> MKSKFKLTTAAAMLGLMVLAGGAQAQDKPREVLTGGHSVSAPQENRIYVMDSVFMHLTESRVHVYDYTNGKFLGMVPTAFNGHVQVSNDGKKIYTMTTYHERITRGKRSDVVEVWDADKLTFEKEISLPPKRVQGLNYDGLFRQTTDGKFIVLQNASPATSIGIVDVAKGDYVEDVTAAAGCWSVIPQPNRPRSFMTICGDGGLLTINLGEDGKVASQSRSKQMFSVKDDPIFIAPALDKDKAHFVSYYGNVYSADFSGDEVKVDGPWSLLNDEDKAKNWVPG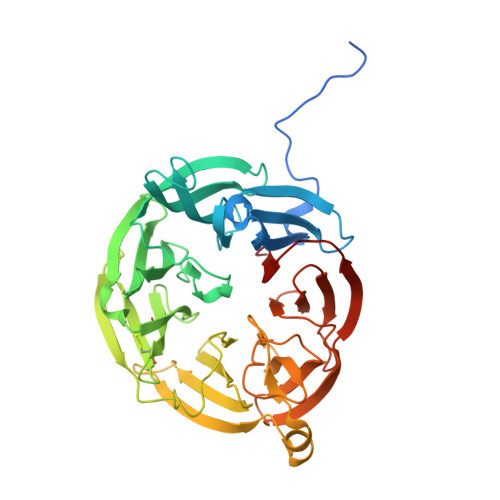GYNLVGLHRASGRMYVFMHPDGKEGTHKFPAAEIWVMDTKTKQRVARIPGRDALSMTIDQQRNLMLTLDGGNVNVYDISQPEPKLLRTIEGAAEASLQVQFHPVGGV> MAHHHHHHVAVDAVSFTLLQDQLQSVLDTLSEREAGVVRLRFGLTDG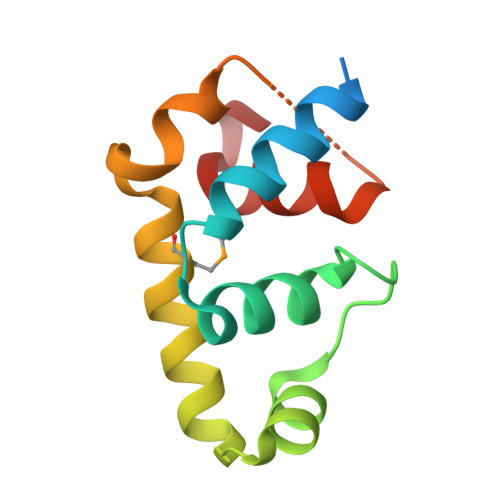QPRTLDEIGQVYGVTRERIRQIESKTMSKLRHPSRSQVLRDYLDGSSGSGTPEERLLRAIFGEKA The stringent response enables bacteria to respond to nutrient limitation and other stress conditions through production of the nucleotide-based second messengers ppGpp and pppGpp, collectively known as (p)ppGpp. Here, we report that (p)ppGpp inhibits the signal recognition particle (SRP)-dependent protein targeting pathway, which is essential for membrane protein biogenesis and protein secretion. More specifically, (p)ppGpp binds to the SRP GTPases Ffh and FtsY, and inhibits the formation of the SRP receptor-targeting complex, which is central for the coordinated binding of the translating ribosome to the SecYEG translocon. Briefly, SRP recognizes hydrophobic signal sequences in the context of translating ribosomes, and SRP bound to ribosome-nascent chain complexes (RNCs) in turn interacts in a GTP-dependent manner with its receptor FtsY, also a GTPase, which localizes at the cytoplasmic membrane periphery of bacteria via a membrane-targeting sequence.

The (Bs)Ffh-NG domain also bound ppGpp and pppGpp with similar affinities as their GDP and GTP counterparts, respectively. We determined the crystal structures of the pppGpp-bound NG domains of (Ec)Ffh and (Ec)FtsY at resolutions of 2.5 and 2.4 Å, respectively, as well as the crystal structures of (Bs)Ffh and (Ec)Ffh in complex with ppGpp and Mg2+ at resolutions of 2.5 and 2.8 Å, respectively. Each of the alarmones could be unambiguously identified by and placed into the available densities. The ppGpp or pppGpp molecules are bound to the G domains of Ffh and FtsY and occupy the canonical guanosine nucleotide-binding site. In detail, the guanine moiety of (p)ppGpp is recognized by the well-described aspartate of the G4 element responsible for the discrimination of guanosine nucleotides by P-loop type GTPases. The α-, β-, and γ-phosphates of (p)ppGpp are coordinated by the G1-element (P-loop), and by residues originating from the switch I and II regions including the G2 and G3 elements, respectively. The δ- and ε-phosphate, which are covalently bound to the 3′-OH group of the ribose moiety and discriminate (p)ppGpp from its GDP/GTP counterparts, point away from the active sites of both GTPases. Both phosphates are not coordinated or form any obvious contacts to the GTPases of Ffh and FtsY. The missing coordination leads to a high flexibility of the δ- and ε-phosphate, as observed in the crystals of (Ec)Ffh with pppGpp. We conclude that ppGpp and pppGpp interact with the SRP-GTPases Ffh and FtsY in the same way as its counterparts GDP and GTP, respectively, also providing the structural explanation for their comparable KD values (see above).

>MGHHHHHHMGFEGLADRLQQTISKIRGKGKVSEQDVKEMMREVRLALLEADVNFKVVKDFVKKVSERAVGQDVMKSLTPGQQVIKVVQEELTELMGGEESKIAVAKRPPTVIMMVGLQGAGKTTTSGKLANLLRKKHNRKPMLVAADIYRPAAIKQLETLGKQLDMPVFSLGDQVSPVEIAKQAIEKAKEEHYDYVILDTAGRLHIDHELMDELTNVKEIANPEEIFLVVDSMTGQDAVNVAKSFNEQLGLTGVVLTKLDGDTRGGAALSIRAVTNTPIKFAGLGEKLDALEPFHPERMASRILGMGDLE[3x]Here we demonstrate that VLPs derived from Cucumber Mosaic Virus can be engineered to incorporate an internally fused Tet-epitope. Vaccines based on the resultant VLPs (CMVTT) are stable, immunogenic, and elicit strong responses even under limiting conditions. CMVTT can easily be linked to any antigen of choice via chemical cross-linking. Cucumber mosaic virus is a widely distributed virus with no toxicity to humans reported to date.

In contrast, replacement of the first 12 N-terminal amino acids of CMV with the TT epitope resulted in well assembled VLPs with a size of approximately 30–40 nm in diameter, as shown by electron microscopy (EM) and dynamic light scattering (DLS), preserving the native T = 3 icosahedral structure. We next characterized the molecular structure of the newly generated CMVTT VLPs by cryoEM. High resolution images were captured and more than 6600 VLPs were picked for averaging, resulting in several 2D classes of VLPs; the best of these were used for 3D- classification. This allowed construction of a 9 Å model, followed by refinement to 4.2 Å, and fitting of the primary sequence into the structure. The structure of CMVTT appeared largely identical to the parent CMV particles (RMSD 1.8 Å), particularly at the surface. Specifically, the subunit arrangement of the asymmetric unit (chains A, B and C) was identical between the parent virus and the modified VLPs. The AA dimers were arranged at the 5-fold axis and the BC dimers around the 3-fold/ pseudo 6-fold axis. Upon closer inspection there were minor differences in the spatial location of the backbone polypeptide in the capsid interior, most likely due to the lack of native viral capsid–genome interactions in the recombinant VLPs. Instead, the modified VLP exhibited additional electron density displaying 3-fold symmetry within the interior cavity (orange color), indicative of novel ordered structures, most likely reflecting tightly bound internal RNA. Interestingly, their relative location and resemblance to tightly-associated RNA species would suggest they might contribute towards stabilizing of intra-subunit associations underlying the overall stability of the particles. A further intriguing aspect of the structure is the relatively large pore size, which may allow for the exchange of naturally bound RNA by other poly-anions or other cargo.

> PGYTFTSITLKPPKIDRGSYYGKRLLLPDSVTEYDKKLVSRLQIRVNPLPKFDSTVWVTVRKVPASSDLSVAAISAMFADGASPVLVYQYAASGVQANNKLLYDLSAMRADIGDMRKYAVLVYSKDDALETDELVLHVDIEHQRIPTSGVLPV;> DANFRVLSQQLSRLNKTLAAGRPTINHPTFVGSERCRPGYTFTSITLKPPKIDRGSYYGKRLLLPDSVTEYDKKLVSRLQIRVNPLPKFDSTVWVTVRKVPASSDLSVAAISAMFADGASPVLVYQYAASGVQANNKLLYDLSAMRADIGDMRKYAVLVYSKDDALETDELVLHVDIEHQRIPTSGVLPV;> ADANFRVLSQQLSRLNKTLAAGRPTINHPTFVGSERCRPGYTFTSITLKPPKIDRGSYYGKRLLLPDSVTEYDKKLVSRLQIRVNPLPKFDSTVWVTVRKVPASSDLSVAAISAMFADGASPVLVYQYAASGVQANNKLLYDLSAMRADIGDMRKYAVLVYSKDDALETDELVLHVDIEHQRIPTSGVLPV> MKAFILAAGSGERLEPITHTRPKAFVPILSKPLIEYQIEYLRKCGIRDITVIVSSKNKEYFEKKLKEISIVTQKDDIKGTGAAILSAKFNDEALIIYGDLFFSNEKEICNIITLKENAIIGVKVSNPKDYGVLVLDNQNNLSKIIEKPEIPPSNLINAGIYKLNSDIFTYLDKISISERGELELTDAINLMAKDHRVKVIEYE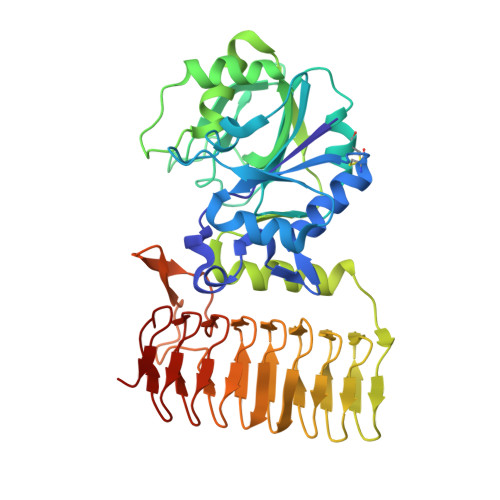GYWMDIGKPWNIIDVNKWALDNLVFSQNLGNVEDNVKIKGKVIIEEDAEIKSGTYIEGPVYIGKGSEIGPNSYLRPYTILVEKNKIGASVEVKESVIMEGSKIPHLSYVGDSVIAEDVNFGAGTLIANLRFDEKEVKVNVKGKRISSGRRKLGAFIGGHVRTGINVTILPGVKIGAYARIYPGAVVNRDVGYGEFFKV Volume-regulated anion channels (VRACs) participate in the cellular response to osmotic swelling. These membrane proteins consist of heteromeric assemblies of LRRC8 subunits, whose compositions determine permeation properties. VRACs are composed of proteins belonging to the conserved LRRC8 family, whose expression is restricted to chordates. This family contains five members in humans, termed LRRC8A–E. All of them share a close sequence relationship and consist of an N-terminal pore domain (PD) followed by a cytoplasmic leucine-rich repeat domain (LRRD). In these assemblies, LRRC8A (or SWELL1) constitutes an obligatory subunit, which is essential for the targeting of channels to the plasma membrane.

Because the binding of Sb1 rigidifies the LRRDs of the four A subunits in the observed conformation, thereby restricting the accessible space of the corresponding domains of the two LRRC8C subunits, we continued to characterize structures of LRRC8A/C in the absence of the sybody. An arrangement closely resembling the LRRC8A/C1:1/Sb1 complex was observed in a dataset of LRRC8A/C obtained in the absence of Sb1. In the 3D reconstruction generated from this dataset, we find a consecutive arrangement of four well-defined subunits that are organized as tightly interacting pairs and two less well-defined subunits. In the latter, additional density at the level of the LRRDs can be attributed to the subunit occupying the C1 position, suggesting that the absence of Sb1 would allow for a better integration of the C subunits in the hexameric protein. However, the LRRDs have rearranged compared to the interactions in the LRRC8A/C/Sb1 complex (by rigid body rotations of 16°, 9°, 11° and 10° for the respective positions A1–A4), leading to a weakening of the tight interface and the creation of a gap between interacting domain pairs. The described movements of the LRRDs of the four A subunits have expanded the accessible space for the respective regions of the adjacent C subunits, as manifested in the emergence of density of the LRRD of the subunit in the C1 position and of the CSD of the less-well-defined C2 position. Remarkably, the relative orientation of the LRRD in the C1 position is distinct from the conformations observed for the A subunits. It instead resembles the arrangement in the LRRC8C heptamer, except for a rigid body rotation by 17° away from the pore axis around a pivot that is located at the interface to the PD. A similar LRRD conformation at the C2 position would result in a clash with the contacted A1 position, requiring a moderate rearrangement that increases the domain mobility, as reflected in its absent density. Considering the observed symmetry mismatch, the incorporation of C subunits and potentially also other LRRC8 homologs into heteromeric channels would perturb the tight interactions found in A homomers and thus destabilize the closed state and improve the activation properties.

>MSIPVTELRYFADTQPAYRILKPWWDVFTDYISIVMLMIAVFGGTLQVTQDKMICLPCKWVTKDSCNDSFRGWAASSPEPTYPNSTVLPTPDTGPTGIKYDLDRHQYNYVDAVCYENRLHWFAKYFPYLVLLHTLIFLACSNFWFKFPRTSSKLEHFVSILLKCFDSPWTTRALSETVVEESDPKPAFSKMNGSMDKKSSTVSEDVEATVPMLQRTKSRIEQGIVDRSETGVLDKKEGEQAKALFEKVKKFRTHVEEGDIVYRLYMRQTIIKVIKFALIICYTVYYVHNIKFDVDCTVDIESLTGYRTYRCAHPLATLFKILASFYISLVIFYGLICMYTLWWMLRRSLKKYSFESIREESSYSDIPDVKNDFAFMLHLIDQYDPLYSKRFAVFLSEVSENKLRQLNLNNEWTLDKLRQRLTKNAQDKLELHLFMLSGIPDTVFDLVELEVLKLELIPDVTIPPSIAQLTGLKELWLYHTAAKIEAPALAFLRENLRALHIKFTDIKEIPLWIYSLKTLEELHLTGNLSAENNRYIVIDGLRELKRLKVLRLKSNLSKLPQVVTDVGVHLQKLSINNEGTKLIVLNSLKKMVNLTELELIRCDLERIPHSIFSLHNLQEIDLKDNNLKTIEEIISFQHLHRLTCLKLWYNHIAYIPIQIGNLTNLERLYLNRNKIEKIPTQLFYCRKLRYLDLSHNNLTFLPADIGLLQNLQNLAVTANRIEALPPELFQCRKLRALHLGNNVLQSLPSRVGELTNLTQIELRGNRLECLPVELGECPLLKRSGLVVEEDLFSTLPPEVKERLWRADKEQALEVLFQ[4x];>[2x]MSIPVTEFRQFSEQQPAFRVLKPWWDVFTDYLSVAMLMIGVFGCTLQVMQDKIICLPKRVQPAQNHSSVPNVSQAVISTTPLPPPKPSPTNPATVEMKGLKTDLDLQQYSFINQMCYERALHWYAKYFPYLVLIHTLVFMLCSNFWFKFPGSSSKIEHFISILGKCFDSPWTTRALSEVSGEDSEEKDNRKNNMNRSGTIQSGPEGNLVRSQSLKSIPEKFVVDKSAAGALDKKEGEQAKALFEKVKKFRLHVEEGDILYAMYVRQTVLKVIKFLIIIAYNSALVSKVQFTVDCNVDIQDMTGYKNFSCNHTMAHLFSKLSFCYLCFVSIYGLTCLYTLYWLFYRSLREYSFEYVRQETGIDDIPDVKNDFAFMLHMIDQYDPLYSKRFAVFLSEVSENKLKQLNLNNEWTPDKLRQKLQTNAHNRLELPLIMLSGLPDTVFEITELQSLKLEIIKNVMIPATIAQLDNLQELCLHQCSVKIHSAALSFLKENLKVLSVKFDDMRELPPWMYGLRNLEELYLVGSLSHDISKNVTLESLRDLKSLKILSIKSNVSKIPQAVVDVSSHLQKMCVHNDGTKLVMLNNLKKMTNLTELELVHCDLERIPHAVFSLLSLQELDLKENNLKSIEEIVSFQHLRKLTVLKLWYNSIAYIPEHIKKLTSLERLFFSHNKVEVLPSHLFLCNKIRYLDLSYNDIRFIPPEIGVLQSLQYFSITCNKVESLPDELYFCKKLKTLKIGKNSLSVLSPKIGNLLFLSYLDIKGNHFEVLPPELGDCRALKRARLVVEDALFETLPSDVREQMKADALEVLFQ> GSLTTISSILSLKREKPDNLAIILQIDFTKLKEEDSLIVVYNSLKALTIKFARLQFCFVDRNNYVLDYGSVLHKIDSLDSISNLKSKSSSTQFSPIWLKNTLYPENI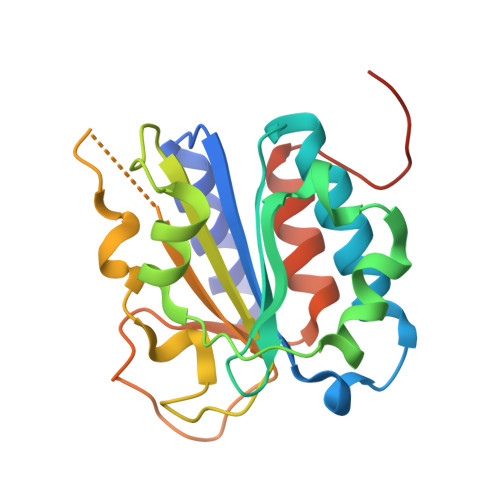HEHLGIVAVSNSNMEAKKSILFQDYRCFTSFGRRRPNELKIKVGYLNVDYSDKIDELVEASSWTFVLETLCYSFGLSFDEHDDDDEEDN> MGWAIVANCEFVNATGKKTTILVNENWAKYCWIWTYKFPEKYTLLRYSVDGEMFMRHRVTFFNATGRYITHTHLNHGLEDVLEGSLAVPK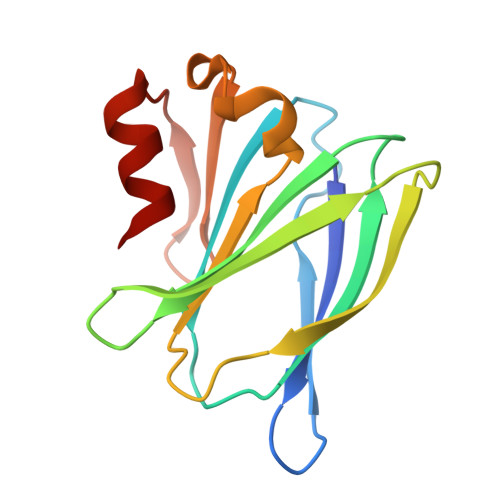DAAYARIHAAINVSLTNPGDVHMHYDETEGEQIRSYDAAEFARTLAAV>MRIPLVGKDSIESKDIGFTLIHEHLRVFSEAVRQQWPHLYNEDEEFRNAVNEVKRAMQFGVKTIVDPTVMGLG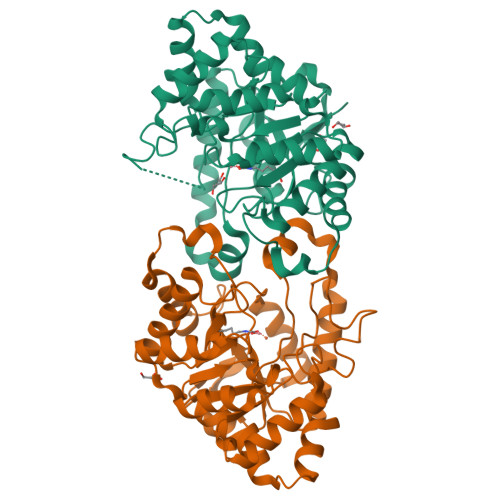RDIRFMEKVVKATGINLVAGTGIYIYIDLPFYFLNRSIDEIADLFIHDIKEGIQGTLNKAGFVKIAADEPGITKDVEKVIRAAAIANKETKVPIITHSNAHNNTGLEQQRILTEEGVDPGKILIGHLGDTDNIDYIKKIADKGSFIGLDRYGLDLFLPVDKRNETTLRLIKDGYSDKIMISHDYLCTFDAGTAKPEYKPKLAPRWSITLIFEDTIPFLKRNGVNEEVIATIFKENPKKFFS[4x]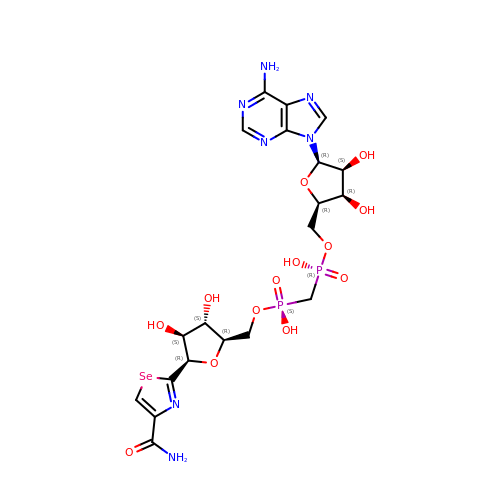BETA-METHYLENE-SELENAZOLE-4-CARBOXYAMIDE-ADENINE DINUCLEOTIDE | C20 H27 N7 O13 P2 Se | BQVYVGJIUMNETO-SFUJTQNPSA-N5-{6-[(1-methylpiperidin-4-yl)oxy]-1H-benzimidazol-1-yl}-3-{[2-(trifluoromethyl)benzyl]oxy}thiophene-2-carboxamide 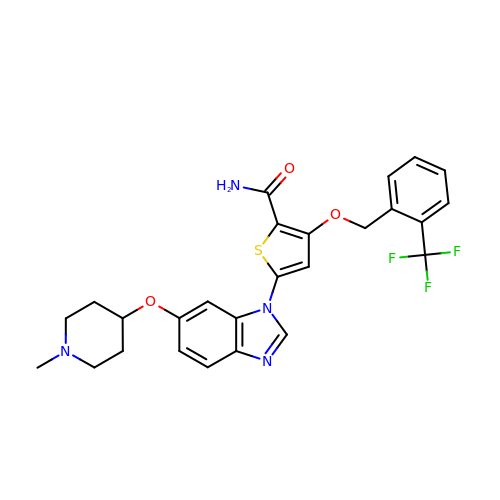| C26 H25 F3 N4 O3 S | FNHUNERGHGEZMB-UHFFFAOYSA-N>[2x]MGSSHHHHHHSQDPSSMTMELRPSGDSGSSDVDAEISDGFSPLDTSHRDVADEGSLLRRAEMYQDYMKQVPIPTNRGSLIPFTSWVGLSISMKQLYGQPLHYLTNVLLQRWDQSRFGTDSEEQRLDSIIHPTKAEATIWLVEEIHRLTPSHLHMALLWRSDPMYHSFIDPIFPEK;>[4x]MADLYPTGQQISFQTTPLNVQDPTRMMNLDQSSPVARNETQNGGGIAHAEFAMFNSKRLESDLEAMGNKIKQHEDNLKFLKSQKNKMDEAIVDLQVHMSKLNSSPTPRSENSDNSLQGEDINAQILRHENSAAGVLSLVETLHGAQASQLMLTKGVVGVVAKLGKVNDENLSQILSNYLGTRSMLAVVCRNYESVTALEAYDNHGNIDINAGLHC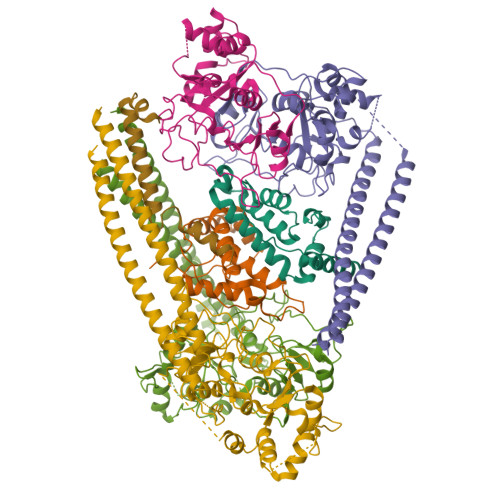LGSSIGREIGDSFDAICLENLRPYVGQHIADDLQRRLDLLKPKLPNGECPPGFLGFAVNMIQIDPAYLLCVTSYGYGLRETLFYNLFSRLQVYKTRADMISALPCISDGAVSLDGGIIRKTGIFNLGNRDEVNVRFAKPTASRTMDNYSEAEKKMKELKWKKEKTLEDIKREQVLREHAVFNFGKKKEEFVRCLAQSSCTNQPMNTPRGTLESGKETAAAKFERQHMDSSTSAA;> GEFFAVSNMLEALDSGKFGSVSKELEEIADMRMDLVKRSIWLYPSLAYTVFEAEKTMDGGGGSDYKDDDDK>[2x]ALVEDNNAVAVSFSEEQEALVLKSWAILKKDSANIA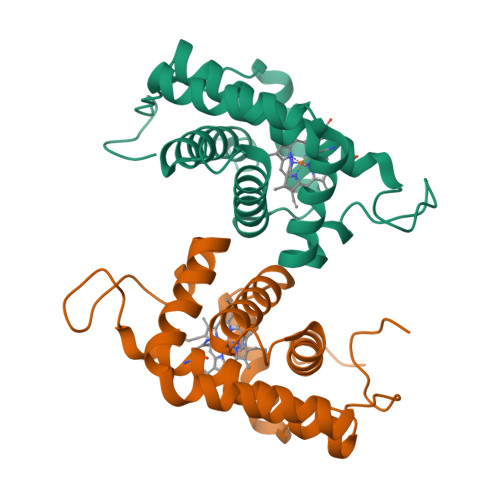LRFWLKIFEVAPSASQMFSFLRNSDVPLEKNPKLKTHAMSVFVMTCEAAAQLRKAGKVTVRDTTLKRLGATHLKYGVGDAHFEVVKFALLDTIKEEVPADMWSPAMKSAWSEAYDHLVAAIKQEMKPAE>[2x]MSDLKVEQVLTSNEWQSTMVTVITDNLPDDTVGPLR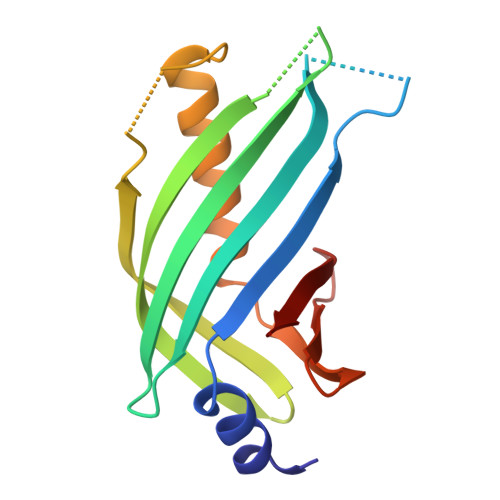RVNVESNVKYLPNGDYIRVSNIKLFAQGSTAESTINISEKGRWEVSDNYLLVSPSEFKDISSSQSKDFSEAQLRLITQIFKLDAEQSRRIDVVNEKTLLLTSLNHGSTVLFRN> GGHMEPLDELDLLLLEEDGGAEAVPRVELLRKKADALFPETVLSRGVDNRYLVLAVETSQNERGAEEKRLHVTASQDREHEVLCILRNGWSSVPVEPGDIVHLEGDCTSEPWIIDDDFGYFILYPDMMISGTSVASSIRCLRRAVLSETFRGSDPATRQMLIGTILHEVFQKAISESFAPERLQELALQTLREVRHLKEMYRLNLSQDEILCEVEEYLPSFSKWAEDFMRKGPSSEFPQMQLSLPSDGSNRSSPCNIEVVKSLDIEESIWSPRFGLKGKIDVTVGVKIHRDCKMKYKVMPLELKTGKESNSIEHRSQVVLYTLLSQERREDPEAGWLLYLKTGQMYPVPANHLDKRELLKLRNWLAASLLHRVSRAAPGEEARLSALPQIIEEEKTCKYCSQIGNCALYSRAVEEQGDDASIPEAMLSKIQEETRHLQLAHLKYFSLWCLMLTLESQSKDNRKTHQSIWLTPASELEESGNCVGNLVRTEPVSRVCDGQYLHNFQRKNGPMPATNLMAGDRIILSGEERKLFALSKGYVKKMNKAAVTCLLDRNLSTLPATTVFRLDREERHGDISTPLGNLSKLMESTDPSKRLRELIIDFREPQFIAYLSSVLPHDAKDTVANILKGLNKPQRQAMKRVLLSKDYTLIVGMPGTGKTTTICALVRILSACGFSVLLTSYTHSAVDNILLKLAKFKVGFLRLGQSHKVHPDIQKFTEEEICRSRSIASLAHLEELYNSHPIVATTCMGINHPIFSRKTFDFCIVDEASQISQPVCLGPLFFSRRFVLVGDHQQLPPLVVNREARALGMSESLFKRLERNESAVVQLTVQYRMNRKIMSLSNKLTYAGKLECGSDRVANAVLALPNLKDARLSLQLYADYSDSPWLAGVLEPDNPVCFLNTDKVPAPEQVENGGVSNVTEARLIVFLTSTFIKAGCSPSDIGVIAPYRQQLRIISDLLARSSVGMVEVNTVDKYQGRDKSLILVSFVRSNEDGTLGELLKDWRRLNVALTRAKHKLILLGSVSSLKRFPPLGTLFDHLNAEQLILDLPSREHESLSHIL

Dna2 has nuclease and helicase activities and plays key roles in maintaining genomic integrity. It is involved in the nucleolytic processing of 5’ flaps during Okazaki fragment maturation, of DNA double-strand breaks (DSBs) during homologous-recombination mediated repair, and of stalled replication forks in the intra-S-phase checkpoint. Dna2 contains a PD-(D/E)XK superfamily nuclease motif and a 5’ to 3’ helicase domain. It is a ssDNA endonuclease that requires a free end for cleavage, and does not cleave dsDNA, single-stranded gaps, D-loops or RNA.

We determined the 2.3 Å crystal structure of full-length mouse Dna2 (residues 1 to 1062) bound to a ssDNA substrate of 21 nucleotides (nts), 15 of which are well ordered. The overall structure has a cylindrical shape with a central tunnel through which the ssDNA threads. The ssDNA is positioned with its 5’ end at the helicase domain, and its 3’ end at the nuclease domain. A 7-nt segment at the 5’ end contacts first the helicase 2A domain outside the tunnel and then the 1A domain inside the tunnel. The DNA crosses over from the helicase to the nuclease domains over the next two nucleotides, which are in the vicinity of the β barrel domain in the middle of the tunnel, but do not make any protein contacts. The subsequent 6-nt segment binds to the nuclease domain. Here, the first three nucleotides are fully enclosed by the tunnel, while the last three nucleotides contact the tunnel opening. The Dna2 nuclease domain binds to a total of four phosphodiester groups, two before and two after the scissile phosphate group. The scissile phosphate group contacts two calcium ions, one (Ca-1) through a non-bridging oxygen, and another (Ca-2) through the 3’ bridging oxygen of the preceding base. The base groups of the 6 nt segment stack in two sets of three, with Met157 and other crossover loop side chains wedging in between the Ade12 and Gua13 base groups.>MLEVVTAGEPLVALVPQEPGHLRGKRLLEVYVGGAEVNVAVALARLGVKVGFVGRVGEDELGAMVEERLRAEGVDLTHFRRAPGFTGLYLREYLPLGQGRVFYYRKGSAGSALAPGAFDPDYLEGVRFLHLSGITPALSPEARAFSLWAMEEAKRRGVRVSLDVNYRQTLWSPEEARGFLERALPGVDLLFLSEEEAELLF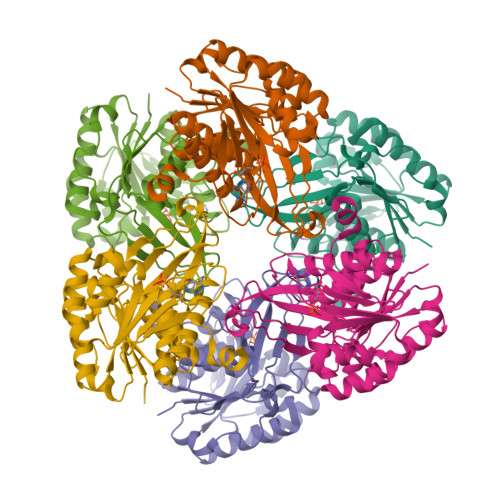GRVEEALRALSAPEVVLKRGAKGAWAFVDGRRVEGSAFAVEAVDPVGAGDAFAAGYLAGAVWGLPVEERLRLANLLGASVAASRGDHEGAPYREDLEVLLKATQTFMR[4x]>[2x]MRGSHHHHHHGLVPRGSGAASGNKATSKGTEEKQDSVRENLDKMISEAEVLNDMAARKLITLDAEQQLELMKSLVATQSQLEATKNLIGDPNATVADLQIAYTTLGNNTQALGNELIKLNPNGQIYAVLNNTEASRAATLRST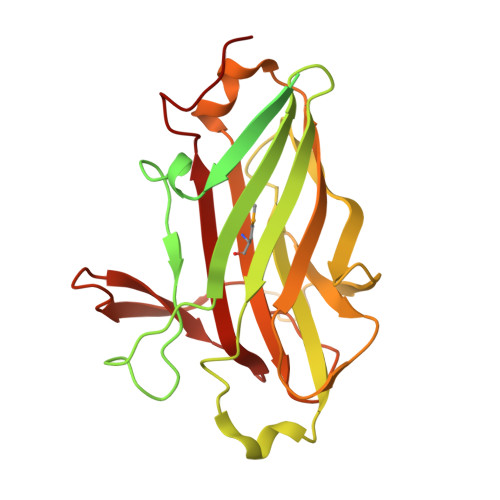TTGTKTTFTISDFSNGGTQYYWAGGNANNLKNPISSISAVYDSATGKISWTVEYDPTTILKSPALKTLKTYTGIYIDTSSDSKLSTPTNVLIDGAATNPVTNFYGNGSKGIEYVSKGTTKGVTKHTITFDTAFSGRANDLADLEIKMLAATTLSDPHFYEDGSKGNYGRYNGQTAPYVIANDSGTAIGGYQVSGVNADSIPSDTT> MAAVFGIQLVPKLNTSTTRRTFLPLRFDLLLDRLQSTNLHGVLYRALDFNPVDRSATVIQTYPPLNAWSPHHAFIENPLDYRDWTEFIHDRALAFVGVLTQRYPLTQNAQRYTNPLVLGAAFGDFLNARSIDIFLDRLFYDPTQDSPITAITKFPYQWTIDSNVTTDSVRTSAGCKYITLYGYDPSRPSTPATYGKHRPTYATVFYYSTLPARSRLLANLAAGPTVLEHFDSPTYGPHLLLPQTGDVLGYSSSLISQAALLMVESVMDALRDNANASASTAVTRLDQSYHPVTSFDPSTFNTLLQRATNLALLAVQGVQSESAIPAIPTMSDVRSFVARLMAEGDPQQWFPYRVDQILYWPESPFVPPIGPFYAPFRPVNFPFTTGSYTVVPDASRPLRLLPQYRNATITVQQADDAYEDTALSPLITTHGFCVTGGVFTSIYDISGDPTAYPPAQLVDAPNDYFDRERMARRDLFRRLRAPADRSAIKDRAVFDFLASLVNPTTANPVLDTSFSMAYLGASSAHANADEPVILADIRSGSIPGLPIPRRIVQFGYDVVHGSLLDLSRAVPTGTFGLVYADLDQVEDAGTDMPAANRAAIAMLGTALQMTTAGGVSVLKVNFPTRAFWTQVFNLYATHATTLHLVKPTIVNSSEVFLVFGGRQSNGALRSTTALQRALLSLYARNAAIDRAVTHIPFFGVPDDGTSDLGIDAVRLFDPMFSDAVANLPSNALASLVSRVVPSSIMFTRVPSNGPVSTTIYGKRTFLSNRRRARLRDVPMLITTTLVHQRRFTTPPTFTLFSSEAVPVTTLVAAGYNSFISEQTRNPNLA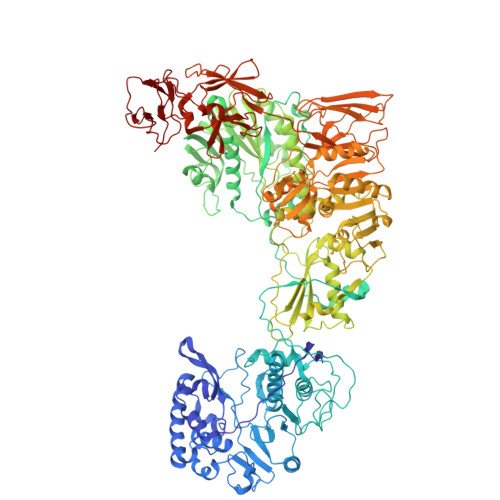HLLDLGTGPECRILSLIPPTLQVTMSDSRPCAELMASFDPALTAYVQGDYSTAAFWNGIRCDSATAIFTIGAAAAAAGTDLIAFVQQLIPRIVAAGGTRMWLQLNTPLYEVSSLPDLIEIDLRDHVYRFNGGERVEPYADPVPLQQAIAALLPAAALSWHTLSPTCDWLPYIIGVGSPLNLSDINTAISYSRLTPILHIDTTTPPLRVNPVPTPLNQQCAIRITSLDPAAVLSVQHNGVEVIGGTPGNVISVAGAAALQYILANQEFLLQFTPTLPGIFDVFLTTLGQPPVPRGSFTITPPPTTVALNMPPPRQLDFTDVGNDARITCDPYYQLAVCIFKDGQYVRVNPEKASVVTNAPNRDLHFVLDLADNHVLLYLCDVTPSGLGDRIAFPIVDIYRIAFPRNTPVRASLPYTGGGAHLTSGGNPFMSLTTPPAVLPAGVALAALSTSVATQYPTYTLPAGVYEYVIE>[2x]MNEALDDIDRILVRELAADGRATLSELAT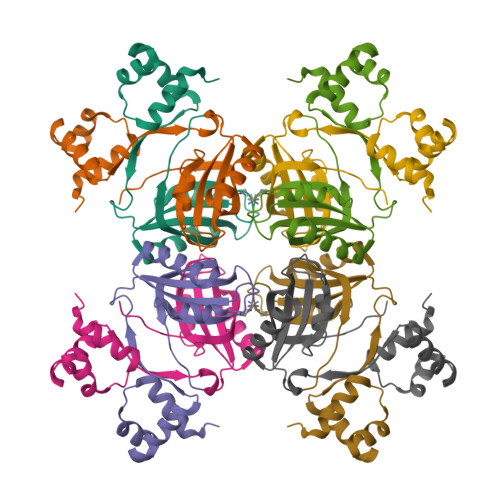RAGLSVSAVQSRVRRLESRGVVQGYSARINPEAVGHLLSAFVAITPLDPSQPDDAPARLEHIEEVESCYSVAGEESYVLLVRVASARALEDLLQRIRTTANVRTRSTIILNTFYSDRQHIP We reconstituted the biosynthesis of the benzoxazole moiety found in nataxazole by adding two enzymes (NatL2, NatAM), to 3‐HAA, ATP, and Mg2+. We have determined the structures of both NatL2 (homologue of BomJ) and NatAM (homologue of BomN) from the antitumor nataxazole pathway. We show NatL2 catalyzes ester not, as previously reported, amide formation; the amide is a shunt product. NatAM catalyzes benzoxazole from this ester by a mechanism that we propose involves shuttling of protons to control the fate of a hemiorthoamide intermediate.

The β‐phosphate of AMPPNP interacts with the side chains of Ser87, Ser88, and Thr239, and backbone amides of Ser88 and Thr239, while the γ‐phosphate has fewer interactions making hydrogen bonds with a water molecule and the side chain of Ser88. There was no electron density for bound Mg2+.

>AMSRSRPELGDWSSPAELAELQRSQLPRVLAQALRSPFYAARYRGTTPPRTADDFAGVEVTAKQDLRDQYPFGMLAVGREHLATYHESSGTAGEPTASYYTEEDWTDLAERFARKWTGIHPSDTFLVRTPYGLVITGHLAQAAGRLRGATVVPGDARSLATPLSRMVRVLKTLDVTLTWCNPTEITMLAAAAKAAGLRPDQDFPHLRAMFTAAEPLTEVRRRRLSEIWGGIPVVEEYGSTETGTIAGQCPEGRMHLWADRAIFEVYDPRTGTLSEAGRGQMVVTPLYRDAMPLLRYNLADDVEVSTDPCGCGWLLPTVTVLGRAGTGHRIGPATVTQQRLEELVFSLPAAYEVMFWRAKAHPDVLELEFEAPEPVRQRAVKELGAALDRELGVPHRITGLAPGTLVPAEALTAQRDILKARYLFAEDEDWDKAVMYF[2x]>MALSANSDAVTYAKAANTRTAAETGDRIEWVKLSLAFLPLATPVSDAKVLTGRQKPLTEVAIIIAEIRSRDGFEGVGFSYSKRAGGQGIYAHAKEIADNLLGEDPNDIDKIYTKLLWAGASVGRSGMAVQAISPIDIALWDMKAKRAGLPLAKLLGAHRDSVQCYNTSGGFLHTPLDQVLKNVVISRENGIGGIKLAVGQPNCAEDIRRLTAVREALGDEFPLMVDANQQWDRETAIRMGRKMEQFNLIWIEEPLDAYDIEGHAQLAA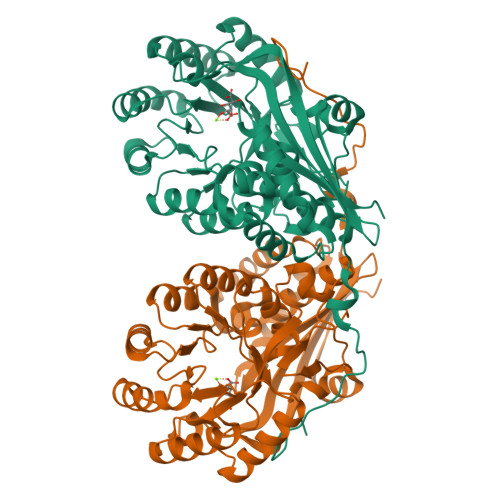ALDTPIATGEMLTSFREHEQLILGNASDFVQPDAPRVGGISPFLKIMDLAAKHGRKLAPHFAMEVHLHLSAAYPLEPWLEHFEWLNPLFNEQLELRDGRMWISDRHGLGFTLSEQARRWTQLTCEFGKRP[3x]>[4x]SNWLIKWDDKFQNDTLSISEFKCSAALAKLGPDPKHPPTKLGEVLNFPHFVAAPEAQTECGSCWKLRYKGNHAFVTVVDRVEEANLF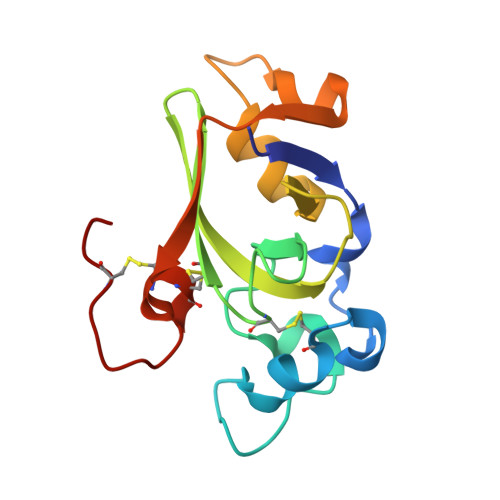VGGTDLVKNLTTFNGAPEGYDWGTAQLFSAYQVDGSCCQQNTGKQCGDP The circadian clock of the cyanobacterium Synechococcus elongatus can be reconstituted in vitro by three proteins, KaiA, KaiB and KaiC. Homo-hexameric KaiC displays kinase, phosphatase and ATPase activities; KaiA enhances KaiC phosphorylation and KaiB antagonizes KaiA. The crystal structure of KaiC from S. elongatus revealed a hexamer in the shape of a double doughnut with approximate dimensions 100×100 Å, whereby the N-terminal CI and C-terminal CII halves of subunits are joined by a 15-amino acid linker. Two phosphorylation sites (P-sites), T432 and S431 that are both located in the CII half were identified in KaiC.

To analyze the phosphorylation patterns of KaiC P-site mutants and to visualize potential conformational variations in the vicinity of bound ATP and residues 432 and 431 at hexamer subunit interfaces, we determined crystal structures of the S. elongatus KaiC single mutants T432A (TSa), S431A (TaT), S431D (TdT), and T426N (nST) and the double mutants T426A/T432A (aSa) and S431A/T432E (Tae). b KaiC mutations xyz or mutants KaiCxyz are sequentially shown in order of sites x = 426, y = 431, and z = 432 where the wild-type residue is in upper case and mutated residues are shown in lower case, i.e. Tsa or KaiCTSa, where the residue at position 426 is T, the residue at position 431 is S, and the residue at position 432 is mutated to A. The crystal structures of the KaiCTaT and KaiCTae mutants are noteworthy in two respects. The structures of the Tae and TaT mutants reveal that T426 residues in some of the six subunits carry a phosphate group and call into question the common assumption of just two P-sites in the core clock protein. Among the structures of the six KaiC mutant proteins reported here, those of the TaT and Tae mutants are the most intriguing because they imply that T426 can be a third phosphorylation site. Therefore, phosphorylation at T426 seen in selected subunits of the Tae and TaT mutants is most likely not a crystallographic artifact. Rather the crystal structures have preserved a third P-site in KaiCII that appears to have evaded identification by other approaches. The T426 phosphorylation site is not a substitute for S431 as demonstrated by the arhythmic behavior of the TaT and aST mutants.

>MTSAEMTSPNNNSEHQAIAKMRTMIEGFDDISHGGLPIGRSTLVSGTSGTGKTLFSIQFLYNGIIEFDEPGVFVTFEETPQDIIKNARSFGWDLAKLVDEGKLFILDASPDPEGQEVVGGFDLSALIERINYAIQKYRARRVSIDSVTSVFQQYDASSVVRRELFRLVARLKQIGATTVMTTERIEEYGPIARYGVEEFVSDNVVILRNVLEGERRRRTLEILKLRGTSHMKGEYPFTITDHGINIFPLGAMRLTQRSSNVRVSSGVVRLDEMCGGGFFKDSIILATGATGTGKTLLVSRFVENACANKERAILFAYEESRAQLLRNAYSWGMDFEEMERQNLLKIVCAYPESAGLEDHLQIIKSEINDFKPARIAIDSLSALARGVSNNAFRQFVIGVTGYAKQEEITGLFTNTSDQFMGAHSITDSHIATITDTIILLQYVEIRGEMSRAINVFKMRGSWHDKAIREFMISDKGPDIKDSFRNFERIISGSPTRITVDEKSELSRIVRGVQEKGPES[6x]> GSHMIARIIGEIGIEGARFIEENIDEQFKALRYLSKGIDSETFVKLVIANSLVSYQLTGKGEQWWWEFAKYFYGRDVKSIYLAYKEFLPNSRFNRRLIPQKLSRIRRVETFLSTLTEERIEEYYGDMSSLWGSIAR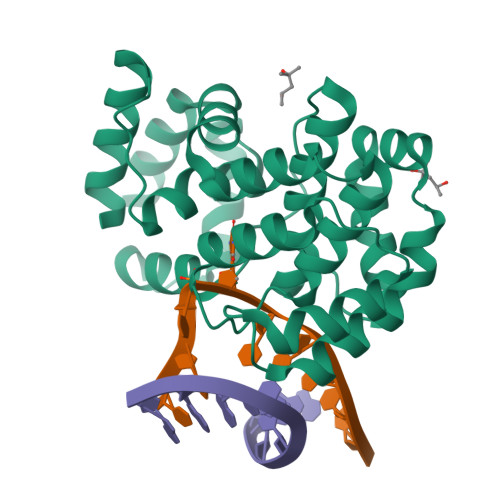ALGVDKESQTVVFSVKMFGYAARIVLSTFNPYPMEIPIPEDSRIVKLTKKLTNEKPRKFWMKIARESGVPPLHIDSILWPLLGGASIDSAPPELRDKLAELIKIIR Metabolite-binding riboswitches are non-coding RNAs that bind to metabolites with high specificity and regulate downstream gene expression in response to changes in metabolite concentrations. S-adenosylmethionine (SAM), a cofactor used in many methylation reactions, is specifically recognized by seven classes of riboswitches, including SAM-I, SAM-II, SAM-III, SAM-IV, SAM-I/IV, SAM-V, and SAM-VI6. Here, we use cryo-EM to determine maps of both apo and ligand-bound SAM-IV riboswitches (119-nt, ~40 kDa) from Mycobacterium sp. to the resolution of 3.7 Å and 4.1 Å, respectively. The SAM-IV riboswitch adopts a double pseudoknot fold involving five helices (P1, P2a, P2b, P3, P5) and two long-range pseudoknot pairings (PK-1, PK-2).

We then decided to record a larger dataset collection on a 300 keV Titan Krios G3 Cryo-Transmission Electron Microscope (Thermo Fisher Scientific) equipped with a Gatan K2 Summit camera without phase plate. A total of ~7000 micrographs were used for further analysis. Compared to the small dataset, the resulting 2D averages and a 3.7-Å 3D reconstruction reveal more detailed RNA features, including all well-resolved major and minor grooves, a traceable sugar phosphate backbone, and some visible base pairs. Supplementary Fig. 2d shows the linear correlation between the particle number and the map resolution, and the B-factor is estimated to be ~219 Å2. To make the RNA model building easier, faster, and more accurate, we used an RNA-specific modeling tool, auto-DRRAFTER to build the initial models for apo and SAM-bound SAM-IV riboswitches, followed by optimization with Phenix18. Starting at the 5’ terminal region of the riboswitch, the ascending strand of P1 with four base pairs is formed. After a turn containing four nucleotides, the riboswitch forms the ascending strand of P2a, followed by one strand of P2b, which is separated by four nucleotides. Following this strand of P2b, C24 to G28 form one strand of the first pseudoknot PK-1. Compared with SAM-I7, SAM-IV lacks the P4 helix but generates a new pseudoknot PK-2 that is connected to the P5 stem-loop. Despite these global differences in the topology of the SAM-I, SAM-I/IV, and SAM-IV structures, all three show at their core two parallel co-axial domains (red and orange) positioned to bind the SAM ligand.

> GGUCAUGAGUGCCAGCGUCAAGCCCCGGCUUGCUGGCCGGCAACCCUCCAACCGCGGUGGGGUGCCCCGGGUGAUGACCAGGUUGAGUAGCCGUGACGGCUACGCGGCAAGCGCGGGUC> MFGRLVLKQTRRTLFNPVLKNTFCIYQAYQNPLRHINTGHNPNNVYEDIVMLGDYPVQNRTHDKVISQTYVPAIANIAFTHLSKKYPQAGLKVDQLNTLKEKTWNDLGVNIEHEKQEILVELSEQIFVKESKLRWVHEQRQRLAHTTYVFSGLEFQNVKVGFFIDSYNFLLQELAHRSNLYQSKDIVGEKSFHEKHLEQQTAPYSGVKSLEEPVSQ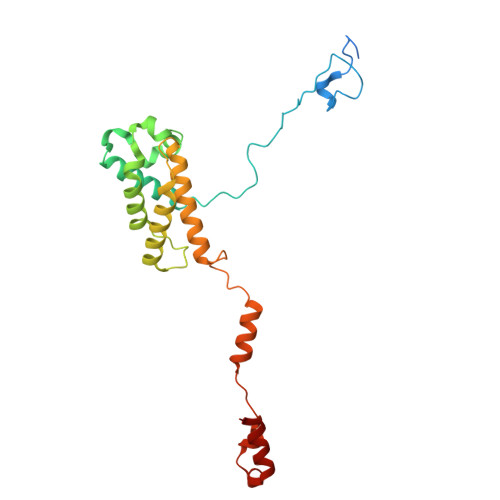NKSFINSLMRAIHNH> MAEYQDKVVDVEVSLGTQPIDTVGFETPMFLAMHGNFPERIRFYVSTAGMVADGFAVGSPAYQFATNAFAGNFAPQRVAIGRMSIDSSKVDFTGTTNTEQVVVNITLNKVVKAVKINVLPGNTPAQIATALADAVTADADLTGKATAVATGTYVTVTAVSPNVVSVGKGAGVYKIVNESSETVATVLPSVIAENHNWYFLATEARSDADIVAAAEFAKANYKLHIYNSTDVDAYAPENSAASVF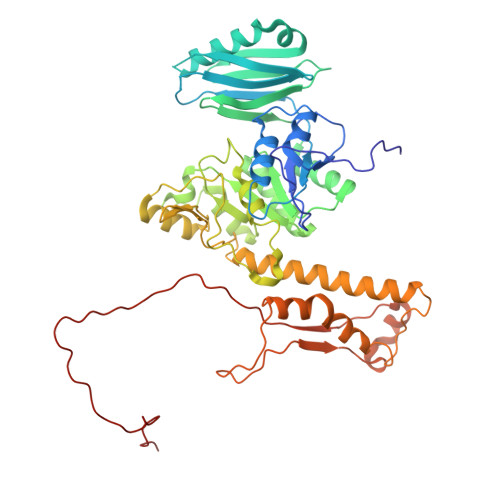DTLKSLSYDSLGTSDAGADVDFTEGSVIGAMAANDPSYGDSLHLKTMPGMVPFAGSDTQRSNAWSRNANIYRGLYGGGSYIEGKTSSGQYVDVIRFSHWVKFRMEESVFAYMKRRSDMGLSMKMSDEDLPVLKSVLMNNPINIGIRNGGILTGYDTENKVSYDPTIIIPKRANIPTNDLAARILRDVKVELVYNNSLHYVKIRASVVLDRPAGQSTNAQTPMSSSAVGV N-[(2S)-3-amino-1-(hydroxyamino)-3-methyl-1-oxobutan-2-yl]-4-[(but-2-yn-1-yl)oxy]benzamide | C16 H21 N3 O4 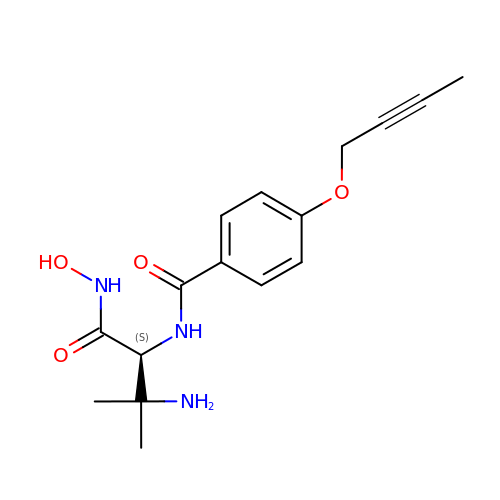| JPCUWLVKAJJSLN-CYBMUJFWSA-N> IDTAAKFIGAGAATVGV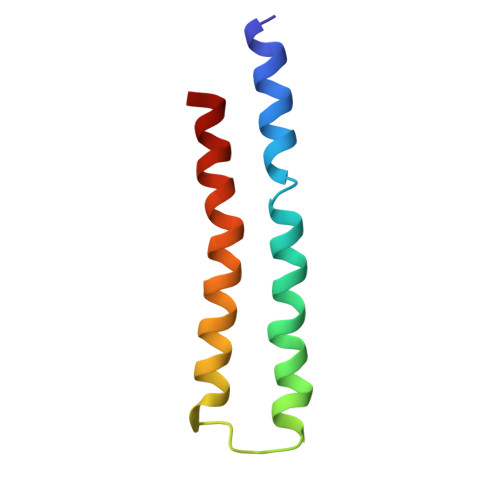AGSGAGIGTVFGSMIIGYARNPSLKQQLFSYAILGFALSEAMGLFCLMVAFLILF>SNTSWRKSEVLAVPLQ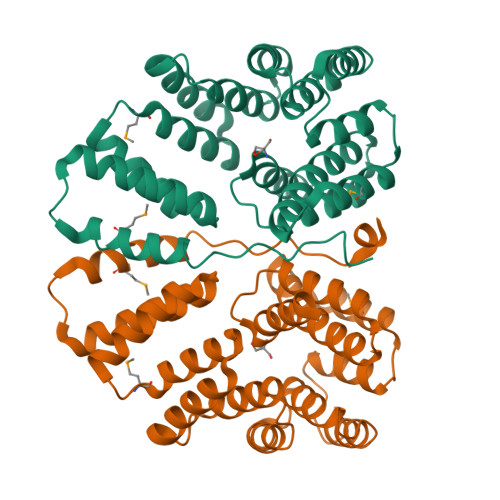PTLQQEVILARMEQILASRALTDDERAQLLYERGVLYDSLGLRALARNDFSQALAIRPDMPEVFNYLGIYLTQAGNFDAAYEAFDSVLELDPTYNYAHLNRGIALYYGGRDKLAQDDLLAFYQDDPNDPFRSLWLYLAEQKLDEKQAKEVLKQHFEKSDKEQWGWNIVEFYLGNISEQTLMERLKADATDNTSLAEHLSETNFYLGKYYLSLGDLDSATALFKLAVANNVHNFVEHRYALLELSLLGQDQDDLAESDQQ[2x]>MAHHHHNSGPLEFTVSANTNPATDAVRESILANPGFGKYYTDHMVSIDYTVDEGWHNAQVIPYGPIQLDPSAIVLHYGQEIFEGLKAYRWADGSIVSFRPEANAARLQSSARRLAIPELPEEVFIESLRQLIAVDEKWVPPAGGEESLYLRPFVIATEPGLGVRPSNEYRYLLIASPAGAYFKGGIKPVSVWLSHEYVRASPGGTGAAKFGGNYAASLLAQAQAAE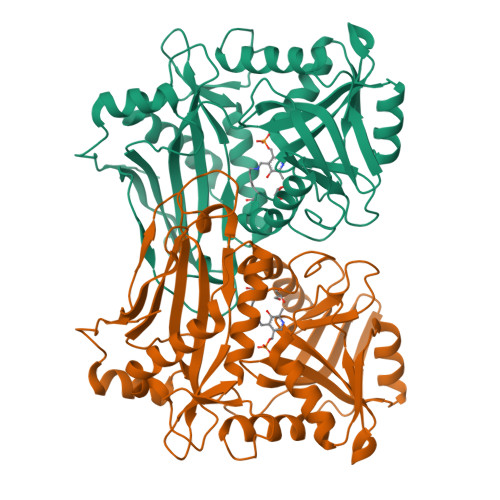MGCDQVVWLDAIERRYVEEMGGMNLFFVFGSGGSARLVTPELSGSLLPGITRDSLLQLATDAGFAVEERKIDVDEWQKKAGAGEITEVFACGTAAVITPVSHVKHHDGEFTIADGQPGEITMALRDTLTGIQRGTFADTHGWMARLN[2x]>[2x]SKAVIVIPARYGSSRLPGKPLLDIVGKPMIQHVYERALQVAGVAEVWVATDDPRVEQAVQAFGGKAIMTRNDH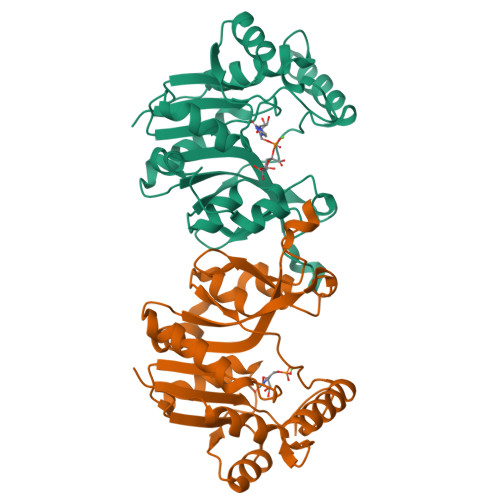ESGTDRLVEVMHKVEADIYINLQGDEPMIRPRDVETLLQGMRDDPALPVATLCHAISAAEAAEPSTVKVVVNTRQDALYFSRSPIPYPRNAEKARYLKHVGIYAYRRDVLQNYSQLPESMPEQAESLEQLRLMNAGINIRTFEVAATGPGVDTPACLEKVRALMAQELAENA> MGSDKIHHHHHHMEKTVIYLLEDGYVDFVVEKIRTKMEKLLEEKDKIFVVLAGGRTPLPVYEKLAEQKFPWNRIHFFLSDERYVPLDSDQSNFRNINEVLFSRAKIPSGNVHYVDT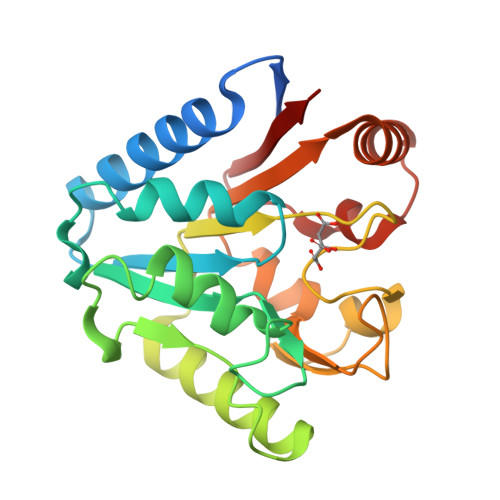SLPIEKACEKYEREIRSATDQFDLAILGMGPDGHVASIFDLETGNKDNLVTFTDPSGDPKVPRVTLTFRALNTSLYVLFLIRGKEKINRLTEILKDTPLPAYFVRGKEKTVWFVGK2-[(1R)-1-{[(E)-azepan-1-ylmethylidene]amino}-2-oxoethyl]-5,5-dimethyl-1,3-thiazolidine-4-carboxylic 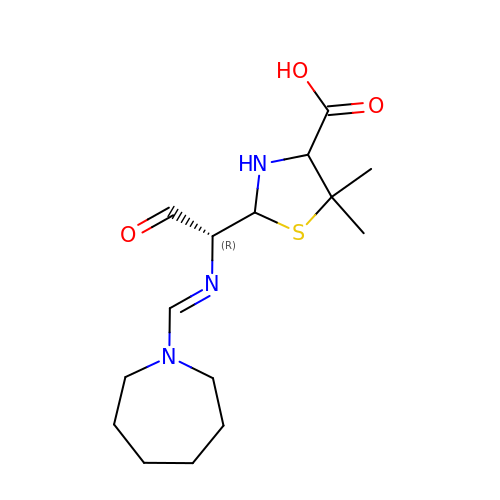acid | C15 H25 N3 O3 S | GIESTXBEHWEDNC-XRSRENSCSA-N> MQEPPD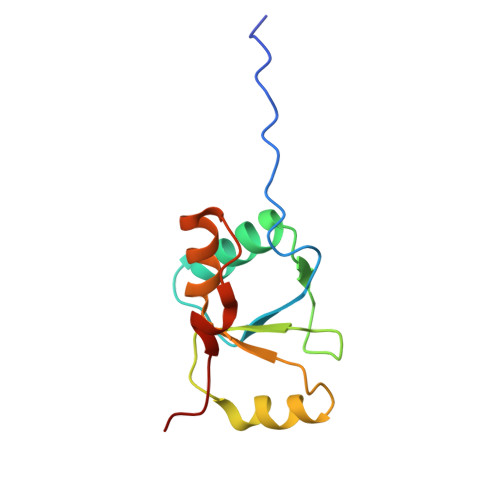LPVPELPDFFEGKHFFLYGEFPGDERRRLIRYVTAFNGELEDRMNERVQFVITAQEWDPNFEEALMENPSLAFVRPRWIYSCNEKQKLLPHQLYGVVPQA4-(4-ethanoylphenyl)-~{N}-[(6-methoxypyridin-3-yl)methyl]piperazine-1-carboxamide 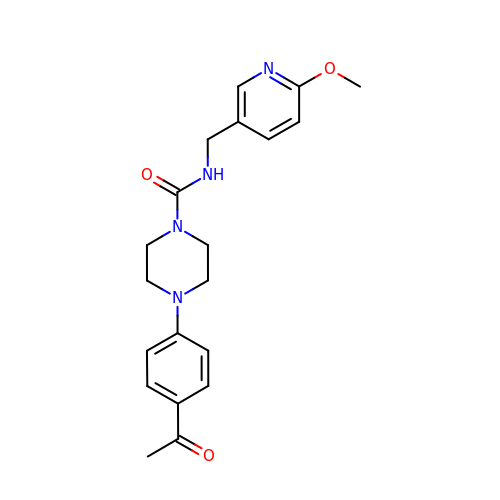| C20 H24 N4 O3 | IWZIKMPFQUSSMX-UHFFFAOYSA-N>SNAGGSSPITGLVYDQRMMLHHNMWDSHHPELPQRISRIFSRHEELRLLSRCHRIPARLATEEELALCHSSKHISIIKSSEHMKPRDLNRLGDEYNSIFISNESYTCALLAAGSCFNSAQAILTGQVRNAVAIVRPPGHHAEKDTACGFCFFNTAALTARYAQSITRESLRVLIVDWDVHHGNGTQHIFEEDDSVLYISLHRYEDGAFFPNSEDANYDKVGLGKGRGYNVNIPWNGGKMGDPEYMAAFHHLVMPIAREFAPELVLVSAGFD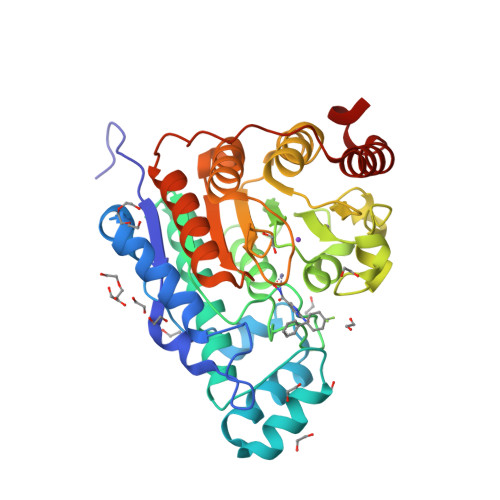AARGDPLGGFQVTPEGYAHLTHQLMSLAAGRVLIILEGGYNLTSISESMSMCTSMLLGDSPPSLDHLTPLKTSATVSINNVLRAHAPFWSSLR[3x]> GPSKMSDVKCTSVVLLSVLQQLRVESSSKLWAQCVQLHNDILLAKDTTEAFEKMVSLLSVLLSMQGAVDINKLCEEMLDNRA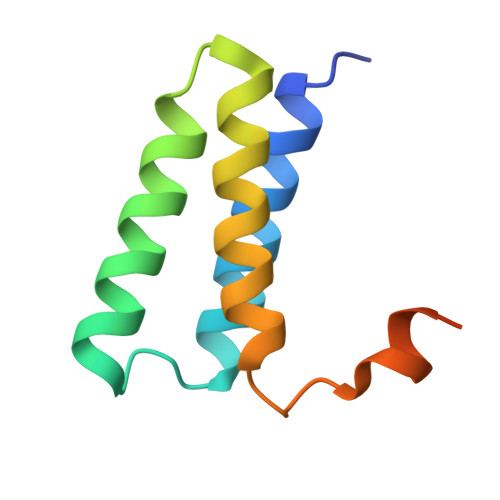TLQ pmcIn neurodegenerative diseases and aging, the microtubule-associated protein tau (MAPT) and the transmembrane lysosomal protein 106B (TMEM106B) become misfolded in different cell types and give rise to intracellular inclusions. TMEM106B aggregates, as discovered using cryo-EM, are composed of amyloid filaments that originate from the carboxy terminus of TMEM106B. The TMEM106B protofilament core spans residues 120–254 and consists of 17 β-strands. We also determined that TMEM106B amyloid filaments were identical in the gray and white matter.

Neuropathologic, biochemical, genetic, and cryo-EM methods were used to study the gray and white matter from the frontal lobes of two individuals affected by multiple system tauopathy with presenile dementia (MSTD). Filaments were made of one or two protofilaments. When a filament was made by two protofilaments, these were identical. Densities corresponding to four asparagine (N) glycosylation sites (N145, N151, N164, and N183) were observed. By whole exome sequencing, it was determined that case #1 was heterozygous for a polymorphism at codon 134 (S134N) of TMEM106B. The encoded residue is inside the protofilament core; however, by cryo-EM, it was not possible to establish whether filaments contained serine or asparagine at position 134 of the core, due to the similarities in the electrodensity of the two residues.

>MGKSLSHLPLHSSKEDAYDGVTSENMRNGLVNSEVHNEDGRNGDVSQFPYVEFTGRDSVTCPTCQGTGRIPRGQENQLVALIPYSDQRLRPRRTKLYVMASVFVCLLLSGLAVFFLFPRSIDVKYIGVKSAYVSYDVQKRTIYLNITNTLNITNNNYYSVEVENITAQVQFSKTVIGKARLNNITIIGPLDMKQIDYTVPTVIAEEMSYMYDFCTLISIKVHNIVLMMQVTVTTTYFGHSEQISQERYQYVDCGRNTTYQLGQSEYLNVLQPQQ[3x]> MPPKKAKGKKKKEEEPDDEYKSMTGADLTQTLEKLKERVNEMRTNRNYIQMDRDMVENFYHNTLKEISEVKTKISNKETEAEEKESKHRIDVKVFLQKVKHLEYEQEKSNLNIEDDGKKAKEKEDAYFEDITKNMKQLKTQLKSEYLEKEKANIQQVQEEKKDHQSLLKIQQKKFDELINNLIIKYEERLAKLKEDLELKLKVEIHELEERKNLHINELMNNHEKAFAELKKYYNDITAENLNLIKAHKEKIAQIYANIQLNTKNVADNQAKNEQLKEPLAKHREIRNKLKEDLKQFAKHKMSLQNLKSKAITLKDKITKLERDGKDLDEKYEKVVREKQELEKKFEDITQEVKKNADLNNNVLSNRLQILLKEYNNKEEELRTIIDNAGLDHNLHEQLKQRVQQSIEAKNTLI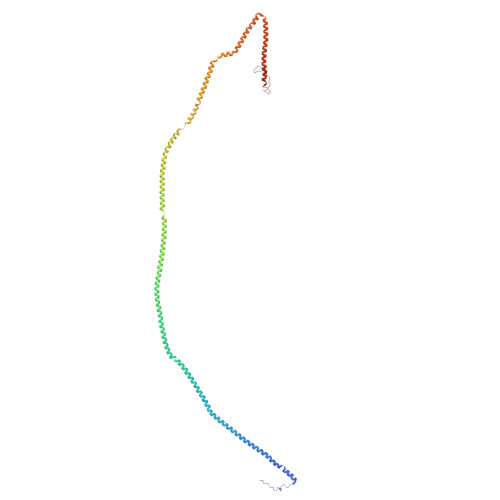KNLKYSIHHATKAYNDAIRVYEAKLVEFGIPIEELGFQPLETITSSMPAGLVSS> MESKGASSCRLLFCLLISATVFRPGLGWYTVNSAYGDTIIIPCRLDVPQNLMFGKWKYEKPDGSPVFIAFRSSTKKSVQYDDVPEYKDRLNLSENYTLSISNARISDEKRFVCMLVTEDNVFEAPTIVKVFKQPSKPEIVSKALFLETEQLKKLGDCISEDSYPDGNITWYRNGKVLHPLEGAVVIIFKKEMDPVTQLYTMTSTLEYKTTKADIQMPFTCSVTYYGPSGQKTIHSEQAVFDIYYPTEQVTIQVLPPKNAIKEGDNITLKCLGNGNPPPEEFLFYLPGQPEGIRSSNTYTLTDVRRNATGDYKCSLIDKKSMIASTAITVHYLDLSLNPSGEVTRQIGDALPVSCTISASRNATVVWMKDNIRLRSSPSFSSLHYQDAGNYVCETALQEVEGLKKRESLTLIVEGKPQIKMTKKTDPSGLSKTIICHVEGFPKPAIQWTITGSGSVINQTEESPYINGRYYSKIIISPEENVTLTCTAENQLERTVNSLNVSAISIPEHDEADEISDENREKVNDQAKLIVGIVVGLLLAALVAGVVYWLYMKKSKTASKHVNKDLGNMEENKKLEENNHKTEA

CD6 is a transmembrane protein with an extracellular region containing three scavenger receptor cysteine rich (SRCR) domains. The membrane proximal domain of CD6 binds the N-terminal immunoglobulin superfamily (IgSF) domain of another cell surface receptor, CD166, which also engages in homophilic interactions. CD6 expression is mainly restricted to T cells, and the interaction between CD6 and CD166 regulates T-cell activation. We have solved the X-ray crystal structures of the three SRCR domains of CD6 and two N-terminal domains of CD166.

Recombinant His-tagged proteins of human CD6 SRCR domains 1–3 and human CD166 IgSF domains 1–3, i.e. the two N-terminal V domains and one C domain (CD166 VVC), were stably expressed in Lec 3.2.8.1 Chinese hamster ovary (CHO) cells, purified, and deglycosylated. Only the first two domains could be resolved in the electron density map. The crystal lattice did not contain space to accommodate the third domain, suggesting it had been proteolytically cleaved prior to crystal growth. We mapped previous mutagenesis data that defined residues in CD166 domain 1 critical for CD6 binding (Skonier et al., 1996a, 1996b) onto the crystal structure. This confirmed the prediction that binding to CD6 is mediated by the AGFCC′C″ face, in common with many other IgSF interactions (Skonier et al., 1996a, 1996b). Mutations in the A′GFCC′C″ face, which disrupt CD6/CD166 interactions, map to the crystal contacts between the two N-terminal domains in the CD166 structure (Bowen et al., 2000). If the heterophilic and homophilic binding sites overlap, as implied by the CD166 crystal contacts, homophilic CD166 interactions would be disrupted by the formation of heterodimers with CD6. Crystal contacts in the CD166 structure suggest that the sites for heterophilic and homophilic binding on CD166 domain 1 overlap.The APOBEC3 family of single-stranded DNA (ssDNA) cytosine deaminases plays important roles in innate immunity against viruses and transposons. However, a subset of APOBEC3 proteins, most notably the nuclear-localized APOBEC3B (A3B) enzyme, is strongly implicated in causing mutations in various human cancers. Human A3B consists of tandem zinc-coordinating cytosine deaminase domains: an N-terminal domain with a pseudo active site and a C-terminal functional catalytic domain. The active site has a catalytically essential zinc ion coordinated by two cysteines (Cys284 and Cys289) and a histidine (His253), with the fourth position of tetrahedral coordination available for directly interacting with the transition state of the hydrolytic cytosine deamination reaction.

The crystals have two protein monomers in the asymmetric unit, each containing a zinc ion bound in the active site. Loops 1 and 7 of A3B(187–378)QM_Δloop3 in the new crystal form show different conformations from those observed previously. In both A and B chains of the new structures, the loop 1 residue Arg211 is flipped out and, instead, the adjacent residue Arg212 projects into the DNA-binding groove and interacts with loop 7 Tyr315. In contrast, Tyr315 in chain B shows an alternative conformation differing by a rotation about the Cα-Cβ bond, in which the Tyr315 side chain is flipped away from loop 1 (χ1 ≈ 180°, trans). Importantly, this trans conformation of Tyr315 was also observed in the open state crystal structure of the A3Bctd active site bound to a TC-containing ssDNA substrate, where the Tyr315 side chain lines a hydrophobic pocket that accommodates the –1 T base. However, in our new apo A3Bctd crystal form, Tyr315 in this alternative conformation maintains the cation-π stacking interaction with the guanidinium group of Arg212. Accordingly, Arg212 in B chain is positioned differently from that in A chain, but is still blocking the ssDNA-binding groove. Of note, the two datasets we collected using different cryo-protectants showed a slight difference in the conformation of Tyr315 in the B chain. In the new crystal form, Arg210 is released and flipped out, replaced by Arg311 that in turn occupies the pocket between α1 and Trp281. The three distinct conformations of the loops 1 and 7 observed in the apo (DNA-free) A3B(187–378)QM_Δloop3 structures collectively represent possible modes of regulated ssDNA access to the A3B active site, in which the closed state of either loop 1 or 7 (or both together) is incompatible with substrate binding.

>SEILRYLMDPDTFTSNFNNDPLVLRRRQTYLCYEVERLDNGTSVKMDQHMGFLCNESGRHAELRFLDLVPSLQLDPAQIYRVTWFISWSPCFSWGCAGEVRAFLQENTHVRLRIKAARIYDYDPLYKEALQMLRDAGAQVSIMTYDEFEYCWDTFVYRQGCPFQPWDGLEEHSQALSGRLRAILQ[2x]>[2x]VSIWSRVVQFGTGWGFWVSGHVFITAKHVAPPKGTEIFGRKPGDFTVTSSGDFLKYYFTSAVRPDIPAMVLENGCQEGVVASVLVKRASGEMLALAVRMGSQAAIKIGSAVVHGQTGMLLTGSNAKAQDLGTIPGDAGCPYVYKKGNTWVVIGVHVAATRSGNTVIAATHGEPTLEALE

Whereas ORF2, ORF3 and ORF4 each encode single proteins, ORF1 codes for a large polyprotein (∼190 kDa) that is processed by the virally-encoded protease at five specific sites to release the six ‘mature’ non-structural proteins (NS1/2–NS7)—and an array of functional precursors—that are required for virus replication. The viral NS6 protease present within the C-terminal half of the polyprotein performs all the processing, including its own autocatalytic release from the precursor (Liu, Clarke & Lambden, 1996; Belliot et al., 2003; Sosnovtsev et al., 2006; Scheffler et al., 2007). Norovirus NS6 is a cysteine protease with a chymotrypsin-like fold: two β-barrel domains separated by a cleft that contains a Cys-His-Asp/Glu catalytic triad similar in arrangement to the Ser-His-Asp triad characteristic of serine proteases. To this end we extended an inactive MNV NS6 construct (which incorporates a C139A mutation to knock out the active site nucleophile) by adding residues from NS7, which is immediately downstream in the polyprotein.

We made three constructs, NS6 1′, NS6 2′ and NS6 4′, which were extended by 1, 2 and 4 residues respectively, generating proteases that contain substrates that correspond to P4–P1′, P4-P2′ and P4-P4′ of the NS6–NS7 cleavage junction. MNV NS6 2′ crystallised in space group P6122 with two molecules in the asymmetric unit. The electron density indicates the positions of residues 3-181 in chain A and 4-181 in chain B, but is not good enough to allow complete modelling of the N- or C-termini. The two monomers found in the asymmetric unit are related by a quasi-2-fold symmetry axis and form an apparent homodimer with an interface area of 1,097 Å2. In addition to neighbourly contacts made by the two C-termini, dimerization within the crystal is stabilised by hydrogen bonds involving Ser 51, Ser 111 and Val 113 of chain A and Ser 51, Ser 52, Ser 111 and Val 113 of chain B. Although the C-termini within the asymmetric unit each embrace the other monomer, reaching into the groove formed between the bII-cII and eII-fII loops, they are again not located within the substrate-binding site. Following anisotropy analysis the MNV NS6 2′ data were truncated to 3.2 Å, 3.2 Å, and 2.7 Å along a∗, b∗ and c∗ directions. The anisotropic truncation of the data, with the new limit of 2.7 Å along the c∗ axis, resulted in a dramatic increase in the number of unique reflections from 8,555 in the “pre-treated” data to 12,786. Anisotropic treatment of the MNV NS6 2′ data also improved the molecular replacement outcome, with a unique solution found by Phaser in contrast with the two possible solutions of the uncorrected data. Nevertheless, this resulted in immediate improvements in refinement: Rwork dropped from 32.5 to 30.3% while Rfree was reduced from 42.0 to 39.0%. These statistics were further improved to Rwork of 25.4% and Rfree of 30.3% in the final structure.>MRILFVAAGSPATVFALAPLATAARNAGHQVVMAANQDMGPVVTGVGLPAVATTDLPIRHFITTDREGRPEAIPSDPVAQARFTGRWFARMAASSLPRMLDFSRAWRPDLIVGGTMSYVAPLLALHLGVPHARQTWDAVDADGIHPGADAELRPELSELGLERLPAPDLFIDICPPSLRPANAAPARMMRHVATSRQC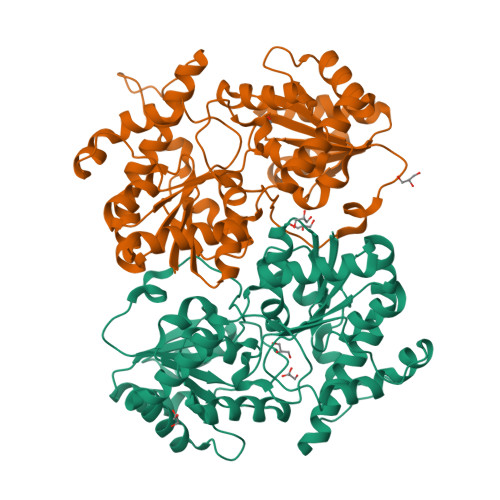PLEPWMYTRDTRQRVLVTSGSRVAKESYDRNFDFLRGLAKDLVRWDVELIVAAPDTVAEALRAEVPQARVGWTPLDVVAPTCDLLVHHAGGVSTLTGLSAGVPQLLIPKGSVLEAPARRVADYGAAIALLPGEDSTEAIADSCQELQAKDTYARRAQDLSREISGMPLPATVVTALEQLAHHHHHH[2x]>DCLSGWSSYEGHCYKAFEKYKTWEDAERVCTEQAKGAHLVSIESSGEADFVAQLVTQNMKRLDFYIWIGLRVQGKVKQCNSEWSDGSSVSYENWIEAESKTCLGLEKETDFRKWVNIYCGQQNPFVCEA[3x];>DCPSDWSSYEGHCYKPFSEPKNWADAENFCTQQHAGGHLVSFQSSEEADFVVKLAFQTFGH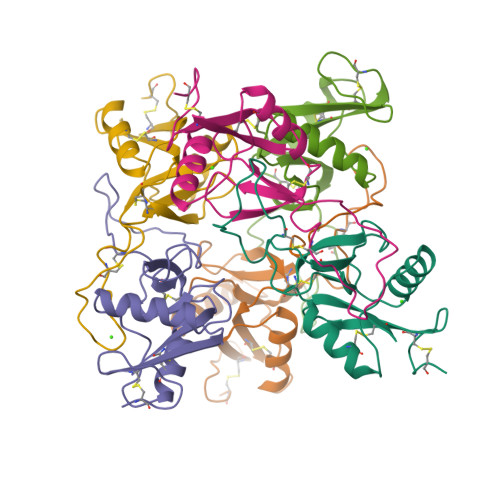SIFWMGLSNVWNQCNWQWSNAAMLRYKAWAEESYCVYFKSTNNKWRSRACRMMAQFVCEFQA[3x]>HHMSEATLLSYTKKLLASPPQLSSTDLHDALLVILSLLQKCDTNSDESLSIYTKVSSFLTALRVTKLDHKAEYIAEAAKAVLRHSDLVDLPLPKKDELHPEDGPVILDIVGTGGDGQNTFNVSTSAAIVASGIQGLKICKHGGKASTSNSGAGDLIGTLGCDMFKVNSSTVPKLWPDNTFMFLLAPFFHHGMGHVSKIRKFLGIPTVFNVLGPLLHPVSHVNKRILGVYSKELAPEYAKAAALVYPGSETFIVWGHVGLDEVSPIGKTTVWHIDPTSSELKLKTFQLEPSMFGLEEHELSKCASYGPKENARILKEEVLSGKYHLGDNNPIYDYILMNTAVLYCLSQGHQNWKEGIIKAEESIHSGNALRSLEHFIDS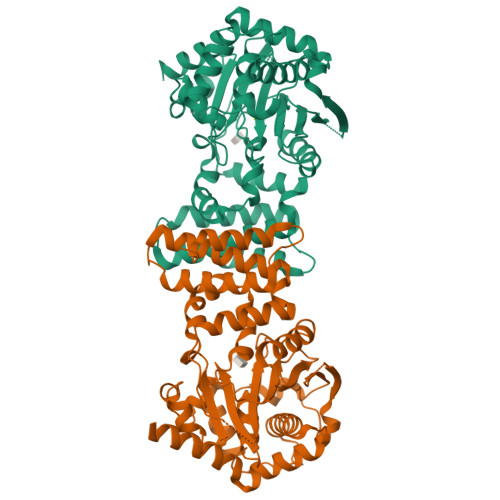VSSL[2x]>SNAAAELRMATTTSTDNTGLLDVLAPAYKKDTGVDLKWVAVGTGNALKLGENCDVDVVFVHAPKVELEYVEKGFGIDRTPVMYNDFVIIGNPSFKQKFTGMSVAEAFKLIEKEQVKFVSRGDKSGTHSKEREVWKEALGKIPEKESWYIEAGQGMLATI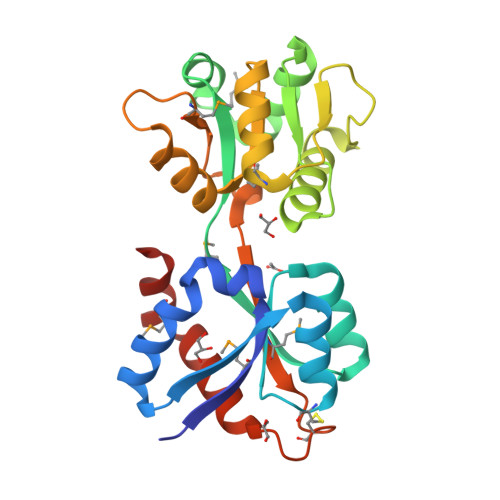NIAEEQKGLTLTDRGTFIKYESNHKGKPPMVIVLEGDNTLKNFYSIMAVNPKRCEKADYKGAKQFIDWIVSEKMQAEIANFKL[3x]4-hydroxy[2,2'-bipyridine]-6-carbaldehyde | C11 H8 N2 O2 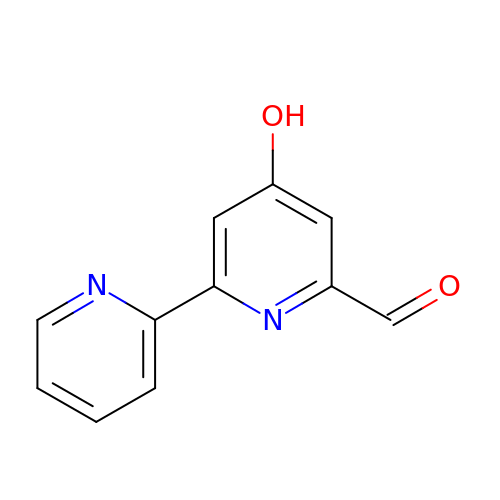| FFOWHRKNAPHKGV-UHFFFAOYSA-N> NKVRTDKKERKRAFPQRGFWKKQNFLQVKNNTVRLAFAVQGVD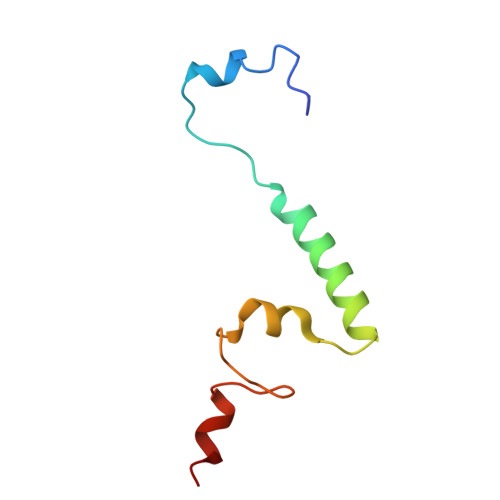LLKLKRLRWGEVRKGNTGWWTDDYRSP> GMPEIHQSIAQHYHERTKYDPETIASKSQRLDWAKQPVPFKEYKIGSAIDLKPYLQETPEVFVNDTNGQWWQRLSRLLFRSYGLTARMPSMGNTVYLRAAPSAGGLYPAEVYVVSRGTPLLSPGLYNYQCRTHSLIHYWESDVWQSLQEACFWHPALESTQLAIIVTAVFYRSAWRYEDRAYRRICLDTGHLLGNIELSAAITDYRPHLIGGFIDEAVNDLLYIDPLQEGAIAVLPLADLLDIQQNISPGCTALPSATETNYPQVPDGELLKYFHHHTQISASITGKLNLPTVIQEKSLEDKYNFPFCLKISTVSAPIYWGENLSDLEITMHKRRSTRAYNGEELTFDELKALLDFTYQPQNYIDQSLDNSPDYFDLNLIETFIAVCGVQGLEAGCYYYAPKAQELRQIRFKNFRRELHFLCLGQELGRDAAAVIFHTSDLKSAIAQYGDRVYRYLHMDAGHLGQRLNLAAIQLNLGVSGIGGFFDDQVNE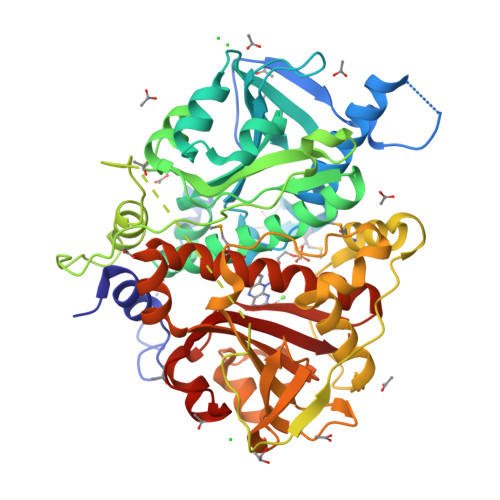VLGIPNDEAVIYITTLGRPR Aerolysin is a β-pore-forming toxin produced by most Aeromonas bacteria, which has attracted large attention in the field of nanopore sensing due to its narrow and charged pore lumen. Pore-forming toxins (PFTs) are important virulence factors of many pathogenic bacteria, which are secreted in a soluble form and upon host membrane binding, they oligomerize into transmembrane pores undergoing a complex structural reorganization. Domains 3 and 4 form the 120 Å long 14-stranded β-barrel, with each protomer contributing two antiparallel β-strands. Four distinct constriction rings, two at each end of the pore, were identified from the structures and confirmed by MD simulation.

In addition, we also solve some key mutants that are regularly used in nanopore experiments, namely, K238A and K238A/K244A. For analyzing the lowest constriction ring, we determined the structure of the K238A/K244A mutant in SMALP obtaining a resolution of 2.2 Å. As expected, the two lysine to alanine mutations also increase the diameter of the lowest two constriction rings without affecting the upper constriction rings. Interestingly, the modification of only K244 leads to a decrease in the lowest constriction, indicating that both K242 and K244 are equally contributing. Also other mutants, such as K238A-K244A, R220A, and T240R, have shown improved sensing capabilities by modifying one of the two constriction sites of the pore. In conclusion, we report high-resolution structures of WT aerolysin along with its K238A and K238A-K244A mutants in SMALPs, amphipols, and LMNG.

>[7x]AEPVYPDQLRLFSLGQGVCGDKYRPVNREEAQSVKSNIVGMMGQWQISGLANGWVIMGPGYNGEIKPGTASNTWCYPTNPVTGEIPTLSALDIPDGDEVDVQWRLVHDSANFIKPTSYLAHYLGYAWVGGNHSQYVGEDMDVTRDGDGWVIRGNNDGGCDGYRCGDKTAIKVSNFAYNLDPDSFKHGDVTQSDRQLVKTVVGWAVNDSDTPQSGYDVTLRYDTATNWSKTNTYGLSEAVTTKNAFKWPLVGETELSIEIAANQSWASQNGGSTTTSLSQSVRPTVPARSKIPVKIELYKADISYPYEFKADVSYDLTLSGFLRWGGNAWYTHPDNRPNWNHTFVIGPYKDKASSIRYQWDKRYIPGEVKWWDWNWTIQQNGLSTMQNNLARVLRPVRAGITGDFSAESQFAGNIEIGAPVPLAA> DHYNC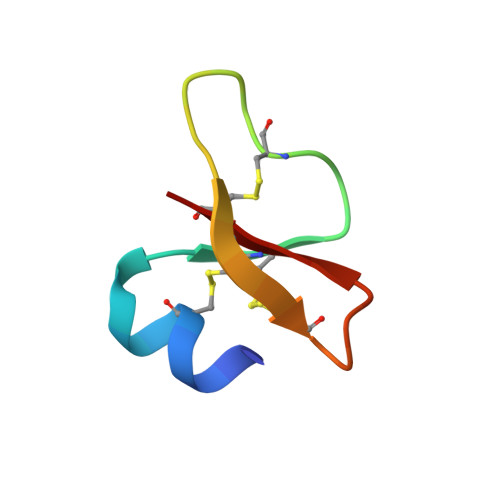VSSGGQCLYSACPIFTKIQGTCYRGEAKCCK>MHHHHHHLPNITILATGGTIAGGGDSATKSNYTVGKVGVENLVNAVPQLKDIANVKGEQVVNIGSQDMNDNVWLTLAKKINTDCDKTDGFVITHGTDTMEETAYFLDLTVKCDKPVVMVGAMRPSTSMSADGPFNLYNAVVTAADKASANRGVLVVMNDTVLDGRDVTMTNTTDVATFKSVNYGPLGYIHNGKIDYQRTPARKHTSDTPFDVSKLNELPKVGIVYNYANASDLPAKALVDAGYDGIVSAGVGNGNLYKSVFDTLATAAKTGTAVVRSSRVPTGATTQDAEVDDAKYGFVASGTLNPQKARVLLQLALTQTKDPQQIQQIFNQY[2x];>MHHHHHHLPNITILATGGDIAGGGDSATKSNYTVGKVGVENLVNAVPQLKDIANVKGEQVVNIGSQDMNDNVWLTLAKKINTDCDKTDGFVITHGTDTMEETAYFLDLTVKCDKPVVMVGAMRPSTSMSADGPFNLYNAVVTAADKASANRGVLVVMNDTVLDGRDVTMTNTTDVATFKSVNYGPLGYIHNGKIDYQRTPARKHTSDTPFDVSKLNELPKVGIVYNYANASDLPAKALVDAGYDGIVSAGVGNGNLYKSVFDTLATAAKTGTAVVRSSRVPTGATTQDAEVDDA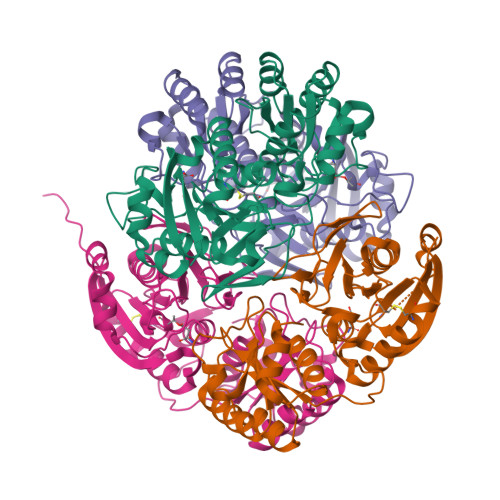KYGFVASGTLNPQKARVLLQLALTQTKDPQQIQQIFNQY[2x]> GSRLCQVDRCTVNLTEAKQYYRRHRVCEVHAKASAATVAGVRQRFCQQCSRFHELPEFDEAKRSCR;>EERVGDMRIVNITFSDINSIKNFQPFSQYFDFTLTGPRYNGNIAQFAMIWKIKNPPHNLLGVFFDNNTRDDEDDKYTLEELKQMGNGAKNMYIFWQYEQK[2x]

SAP05 is an effector from a plant pathogenic phytoplasma that mediates the degradation of host transcription factors, including SPL and GATA family proteins, by hijacking the 26 S plant ubiquitin receptor RPN10 independently of substrate ubiquitination. Specifically, SAP05 folds into a tight globular structure consisting of a parallel five-stranded β-sheet (β1-β5). Although SAP05 carries a single domain, it utilizes two opposing surfaces (hereafter referred to as Lobe1 and Lobe2) to interact simultaneously with TFs and AtRPN10, forming a dumbbell-shaped structure, in which TFs and AtRPN10 have no direct surface contacts. In summary, SAP05 bridges the TFs mainly through electrostatic interactions with a hydrophobic core, whereas the SAP05-AtRPN10 interface comprises predominantly extensive hydrophobic contacts.

In the SAP05-SPL5 binary complex, the ZnF of SPL5 possesses two zinc-binding subdomains, of which N-terminal subdomain contains an extended loop followed by two short helices to coordinate one Cys3His-type zinc finger motif, whereas the C-terminal subdomain employs a three-stranded antiparallel β-sheet and a short helix to coordinate a Cys2HisCys-type zinc finger motif. It should be noted that, unlike other types of zinc-binding domains, these two zinc-binding sequence motifs are not interleaved, thereby forming a unique plant-specific TF called SQUAMOSA promoter binding protein (SBP). In the SAP05-SPL5 structure, both subdomains of SPL5 participate in the interactions with SAP05. Particularly, for the N-terminal subdomain’s contacts, a hydrophobic core is formed at the interface between the α1 of the N-terminal subdomain donated by Tyr78 and Tyr79 and the β3 of SAP05 donated by Ile84 and Trp85. Besides, the Lys90 from α2 of the N-terminal subdomain forms a bidentate salt bridge with the carboxyl group of Glu107 from SAP05. Likewise, for the C-terminal subdomain’s contacts, a bidentate salt bridge is created by the Arg121 and the Asp106. This interface is further strengthened by three direct hydrogen bonds contributed by Gln105 and Ser108 of the C-terminal subdomain with Arg104 and Asn77 of SAP05. For example, in the SAP05-SPL5 interface, substitution of SAP05 Glu107 or Asp106 with alanine, which would disrupt the salt-bridged interaction, resulted in 15-fold decreased or abolished binding affinity for SPL5. Moreover, the alanine substitution of SAP05 Trp85, impairing hydrophobic interaction, caused a complete loss of SPL5 binding. In parallel, alanine replacement of the corresponding electrostatic or hydrophobic interacting Arg121, Tyr78 or Tyr79 in SPL5 abrogated its ability to bind SAP05.> SHMLSREDNELLVRVGPGTAMGTMMRLYWIPFLKSSEVTAGGQPYRVRLLGEDLVAFRDNSGNVGLVDHTCPHRGAPMVFGRNENDGLRCVYHGWKFKVSGQCEEMPCEPADSPMCKRMKIKAYPVKERNGILWAYMGPDAENAPELPDVEWNMVPEEQVAISMRVQECNWLQALEGELDSAHAAILHGRVGEGGVINQWRQAQDLSPTF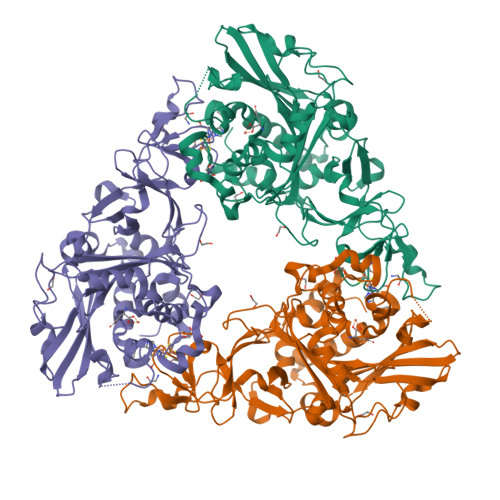ECVQHDAGISIGARRKTPDGENYVRVNQFLMPFWTLVPPQSQFPELSGHAWVPIDDEHTLCLMFSYHPAKPFYERTRKLFKEGHNGRETGHHSDNAFEKRPVTEPYHTYWSKFNRGNAYQFDYQSQVEKYNSGMPGLWIQDAACQSGTTPILDRSKEHLGTSDTGVARMRRVLLEAVKKLVATGEHPVSSNAPAAFRWRAVSLTIPLGGDWTKLGEEAMRAEPGKDFGYTP2-methyl-2-{[(3-methylthiophen-2-yl)methyl]amino}propan-1-ol 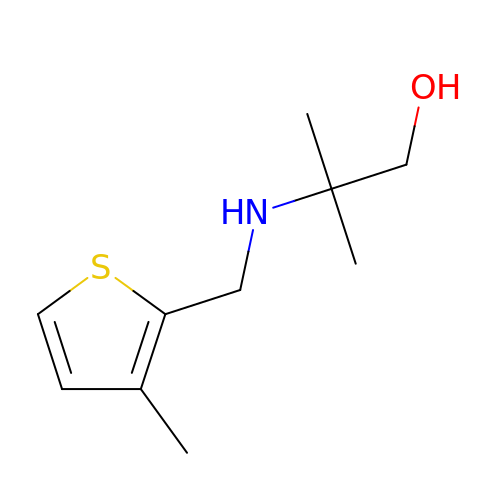| C10 H17 N O S | IFQLAGXBYFTXBB-UHFFFAOYSA-N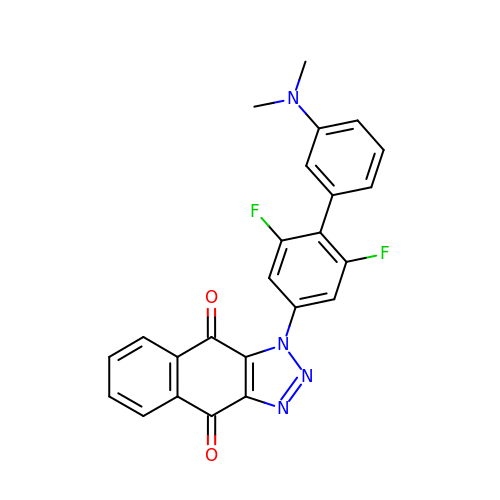3-[4-[3-(dimethylamino)phenyl]-3,5-bis(fluoranyl)phenyl]benzo[f]benzotriazole-4,9-dione | C24 H16 F2 N4 O2 | DIQAKQHNMJSKDT-UHFFFAOYSA-N> EVYALEESRDVYLSDLDWLNATHGDDTKSKIVQKNHPFTPGNNNQSTKISLKMEDGSISEFEKGLGTIAGSPSTITYDISGAGVTK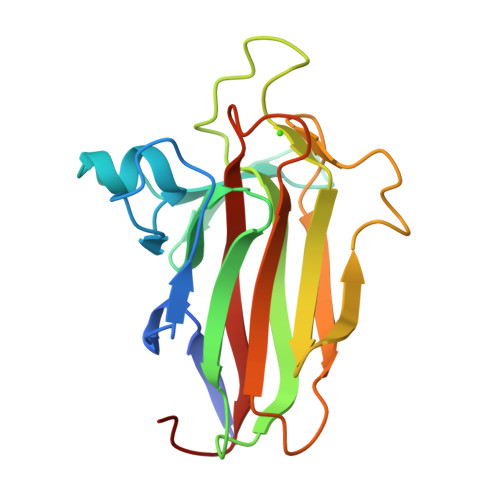FFSYLGIDRSANPINEQYAKVDKIEVVVDGKVIYSTINQFPNGLTYETPAIKVDLNIPENAKRLQLKSYAGEKTWGDEVVYADAKFTAKGDFVN> MSGKDRIEIFPSRMAQTIMKARLKGAQTGRNLLKKKSDALTLRFRQILKKIIETKMLMGEVMREAAFSLAEAKFTAGDFSTTVIQNVNKAQVKIRAKKDNVAGVTLPVFEHYH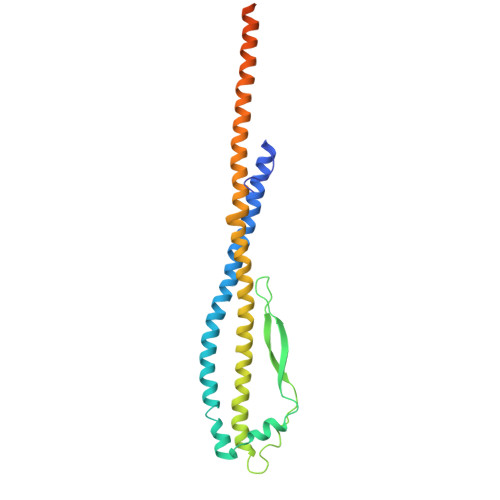EGTDSYELTGLARGGEQLAKLKRNYAKAVELLVELASLQTSFVTLDEAIKITNRRVNAIEHVIIPRIERTLAYIITELDEREREEFYRLKKIQEKKKILKEKSDKDLEQRRAAGEVIEPANLLAEEKDEDLLFE>[3x]MRGSHHHHHHGIR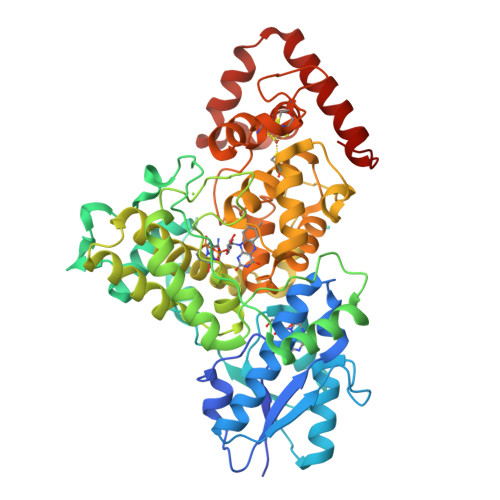MLTRLILVLGDQLSDDLPALRAADPAADLVVMAEVMEEGTYVPHHPQKIALILAAMRKFARRLQERGFRVAYSRLDDPDTGPSIGAELLRRAAETGAREAVATRPGDWRLIEALEAMPLPVRFLPDDRFLCPADEFARWTEGRKQLRMEWFYREMRRRTGLLMEGDEPAGGKWNFDTENRKPAAPDLLRPRPLRFEPDAEVRAVLDLVEARFPRHFGRLRPFHWATDRAEALRALDHFIRESLPRFGDEQDAMLADDPFLSHALLSSSMNLGLLGPMEVCRRAETEWREGRAPLNAVEGFIRQILGWREYVRGIWTLSGPDYIRSNGLGHSAALPPLYWGKPTRMACLSAAVAQTRDLAYAHHIQRLMVTGNFALLAGVDPAEVHEWYLSVYIDALEWVEAPNTIGMSQFADHGLLGSKPYVSSGAYIDRMSDYCRGCAYAVKDRTGPRACPFNLLYWHFLNRHRARFERNPRMVQMYRTWDRMEETHRARVLTEAEAFLGRLHAGEPV> MSLRVILFDLDGTLIDSAKDIALALEKTLKELGLEEYYPDNVTKYIGGGVRALLEKVLKDKFREEYVEVFRKHYLENPVVYTKPYPEIPYTLEALKSKGFKLAVVSNKLEELSKKILDILNLSGYFDLIVG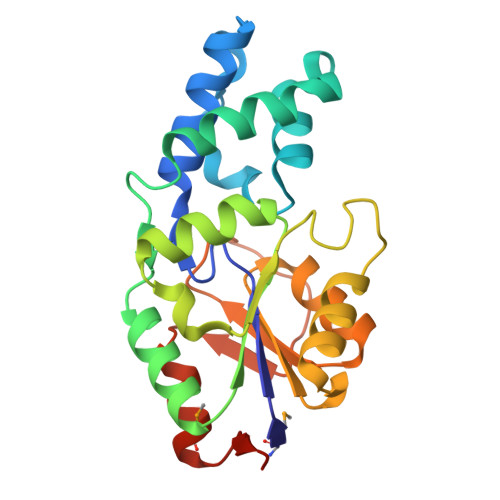GDTFGEKKPSPTPVLKTLEILGEEPEKALIVGDTDADIEAGKRAGTKTALALWGYVKLNSQIPDFTLSRPSDLVKLMDNHIVEFEGHHHHH>RSPWPGFSDETLDKVPKSEGYCSRILRAQGTRREGYTEFSLRVEGDPDFYKPGTSYRVTLSAAPPSYFRGFTLIALRENREGDKEEDHAGTFQIIDEEETQFMSNCPVAVTESTPRRRTRIQVFWIAPPAGTGCVILKASIVQKRIIYFQDEGSLTKKLCEQDSTFDGV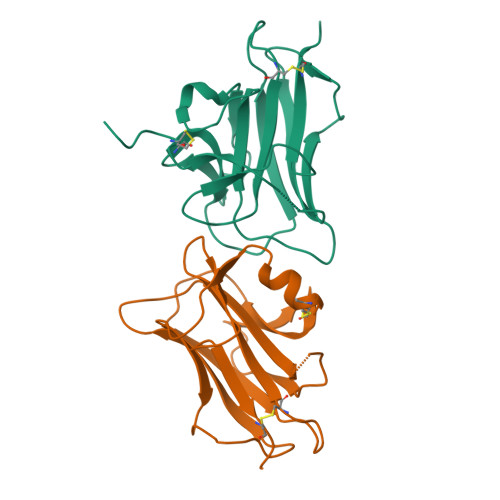TDKTGHHHHHH[2x]Monopolar spindle 1 (Mps1) is a dual‐specificity protein kinase, orchestrating faithful chromosome segregation during mitosis. Mps1 acts as a master conductor of SAC signaling by phosphorylating various kinetochore components. The Mps1 kinase domain adopts the canonical kinase architecture with an N‐terminal lobe connected with a hinge loop to the C‐terminal lobe that contains the catalytic loop, the activation loop, and the P + 1 loop. All reported structures of the Mps1 kinase adopt the hallmarks of an inactive conformation, which includes a mostly disordered activation loop.

To investigate whether the MDS region is interfering with the kinase domain structurally, we then crystallized Mps1400‐808 in the presence of ATP. The crystal structure was determined by molecular replacement, at 2.4 Å resolution (Table 1 and Figure 1C−E). However, the electron density did not show any likely placement for the MDS region, suggesting it is either very flexible or degraded during crystallization. Notably, neither ATP nor its hydrolysis product ADP was observed in the ATP binding pocket. To our surprise however, while inspecting the structure we noticed that unambiguous density was present for residues 670‐685, the activation loop of the Mps1 kinase. The activation loop has a random coil structure except residues 677‐680 that form a single helical turn. It should be noted that the observed conformation of the activation loop is stabilized by crystallographic contacts. However, the observed conformation of the loop, which is affected by crystal contacts, blocks access to the ATP binding pocket, and the kinase remains in the inactive conformation. The conserved acidic residue, Glu 571 in the αC helix, does not form a salt bridge with the catalytic Lys 553, which in turn stabilizes the ATP binding; instead, the backbone nitrogen atoms of activation loop residues, Phe 665, Ile 667, and Ala 668 make a hydrogen bonding network with Glu 571. In the current structure, the hydrophobic R‐spine is disassembled, also suggesting that our structure is in an inactive conformation.

> MAHHHHHHSAALEVLFQGPGPAASSNHWQIPELARKVNTEQKHTTFEQPVFSVSKQSPPISTSKWFDPKSICKTPSSNTLDDYMSCFRTPVVKNDFPPACQLSTPYGQPACFQQQQHQILATPLQNLQVLASSSANECISVKGRIYSILKQIGSGGSSKVFQVLNEKKQIYAIKYVNLEEADNQTLDSYRNEIAYLNKLQQHSDKIIRLYDYEITDQYIYMVMECGNIDLNSWLKKKKSIDPWERKSYWKNMLEAVHTIHQHGIVHSDLKPANFLIVDGMLKLIDFGIANQMQPDTTSVVKDSQVGTVNYMPPEAIKDMSSSRENGKSKSKISPKSDVWSLGCILYYMTYGKTPFQQIINQISKLHAIIDPNHEIEFPDIPEKDLQDVLKCCLKRDPKQRISIPELLAHPYVQIQTHPVNQMAKGTTEE> GTDAPTEAALKAERTFMAGEKAKPGVKELADGILMTELTPGTGPKPDANGRVEVRYVGRLPDGKIFDQSTQPQWFRLDSVISGWTSALQNMPTGAKWRLVIPSDQAYGAEGAGDLIDPFTPLVFEIE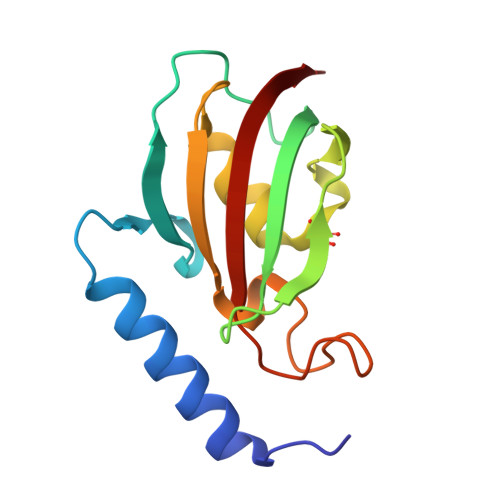LIAVSQ> GEAPADRLKALVDAAVQPVMKANDIPGLAVAISLKGEPHYFSYGLASKEDGRRVTPETLFEIGSVSKTFTATLAGYALTQDKMRLDDRASQHWPALQGSRFDGISLLDLATYTAGGLPLQFPDSVQKDQAQIRDYYRQWQPTYAPGSQRLYSNPSIGLFGYLAARSLGQPFERLMEQQVFPALGLEQTHLDVPEAALAQYAQGYGKDDRPLRVGPGPLDAEGYGVKTSAADLLRFVDANLHPERLDRPWAQALDATHRGYYKVGDMTQGLGWEAYDWPISLKRLQAGNSTPMALQPHRIARLPAPQALEGQRLLNKTGSTNGF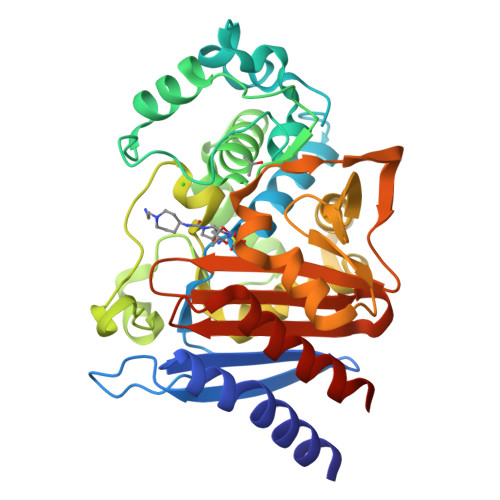GAYVAFVPGRDLGLVILANRNYPNAERVKIAYAILSGLEQQGKVPLKA5-hydroxydiclofenac | C14 H11 Cl2 N O3 | 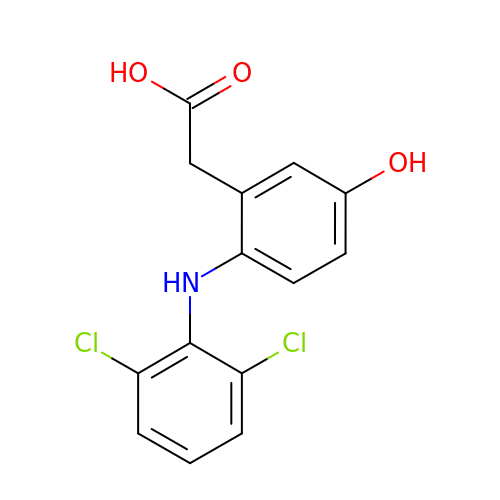VNQURRWYKFZKJZ-UHFFFAOYSA-N Macrolide resistance is abundant in pathogenic bacteria, and is most often the result of GTP-dependent macrolide kinases (Mph), ribosomal methyltransferases, or efflux pumps. Mph enzymes inactivate macrolides by phosphorylating the 2′-OH of the essential dimethylamino sugar, preventing it from binding the ribosome, and providing the chemical rationale for the resistance phenotype. Mph enzymes are therefore adaptable resistance enzymes with complex evolutionary paths.

While the MphA, MphB, and MphH structures are very similar, we observed structural distinctions in all three enzymes that localized to the (a) NPL, (b) β-hairpin insert, and (c) multiple residues in the macrolide-binding cleft. Consistent with the flexibility of MphH in our crystal structure, these observations highlight that conformational changes in these key regions of Mph enzymes play a role in macrolide substrate binding.

> GMPEDLDALLDLAARHGLDLDGGTLRTEEIGLDFRVAFARAHDGGDWVLRLPRRPDVLERAAVEGRLLAMLAPHLDVAVPDWRISTSELIAYPLLPGSPGLTVAADGEVSWHVDMASTVYARSLGSVVAQLHAVDAEAAAATGIEVRSPAQVRGAWRQDLARVGAEFEIAPALRERWEAWLADDGCWPGHSVLTHGELYPAHTLVEDERITAVLDWTTAAVGDPAKDLMFHQVSAPSAIFEVALQAYAEGGGRPWPGLARHCTEMFSAAPLGYGLYALATGEAAHREAAAAALNPPEER>[2x]METFDPTELPELLKLYYRRLFPYSQYYRWLNYGGVIKNYFQHREFSFTLKDDIYIRYQSFNNQSDLEKEMQKMNPYKIDIGAVYSHRPNQHNTVKLGAFQAQEKELVFDIDMTDYDDVRRCCSSADICPKCWTLMTMAIRIIDRALKEDFGFKHRLWVYSGRRGVHCWVCDESVRKLSSAVRSGIVEYLSLVKGGQDVKKKVHLSEKIHPFIRKSINIIKKYFEEYALVNQDILENKESWDKILALVPETIHDELQQSFQKSHNSLQRWEHLKKVASRYQNNIKNDKYGPWLEWEIMLQYCFPRLDINVSKGINHLLKSPFSVHPKTGRISVPIDLQKVDQFDPFTVPTISFICRELDAISTNEEEKEENEAESDVKHRTRDYKKTSLAPYVKVFEHFLENLDKSRKGELLKKSDLQKDF;>[2x]MEFSGRKWRKLRLAGDQRNASYPHCLQFYLQPPSENISLIE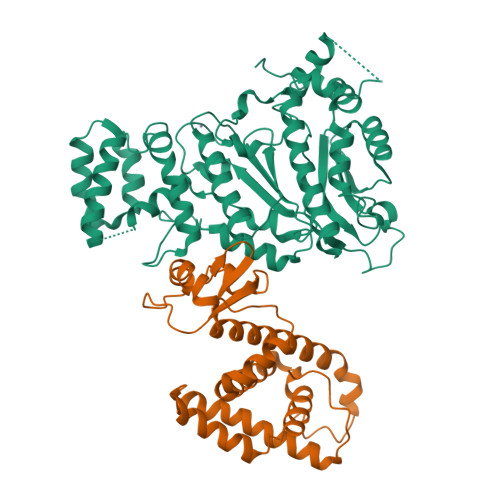FENLAIDRVKLLKSVENLGVSYVKGTEQYQSKLESELRKLKFSYRENLEDEYEPRRRDHISHFILRLAYCQSEELRRWFIQQEMDLLRFRFSILPKDKIQDFLKDSQLQFEAISDEEKTLREQEIVASSPSLSGLKLGFESIYKIPFADALDLFRGRKVYLEDGFAYVPLKDIVAIILNEFRAKLSKALALTARSLPAVQSDERLQPLLNHLSHSYTGQDYSTQGNVGKISLDQIDLLSTKSFPPCMRQLHKALRENHHLRHGGRMQYGLFLKGIGLTLEQALQFWKQEFIKGKMDPDKFDKGYSYNIRHSFGKEGKRTDYTPFSCLKIILSNPPSQGDYHGCPFRHSDPELLKQKLQSYKISPGGISQILDLVKGTHYQVACQKYFEMIHNVDDCGFSLNHPNQFFCESQRILNGGKDIKKEPIQPETPQPKPSVQKTKDASSALASLNSSLEMDMEGLEDYFSEDS> APIRVVSVPESDSFMSSVPDNSTPLYPKVVVPPRQVPGRFTNFIDVAKQTYSFCSISGKPYFEVTNTSGDEPLFQMDVSLSAAELHGTYVASLSSFFAQYRGSLNFNFIFTGAAATKAKFLVAFVPPHSAAPKTRDEAMACIHAVWD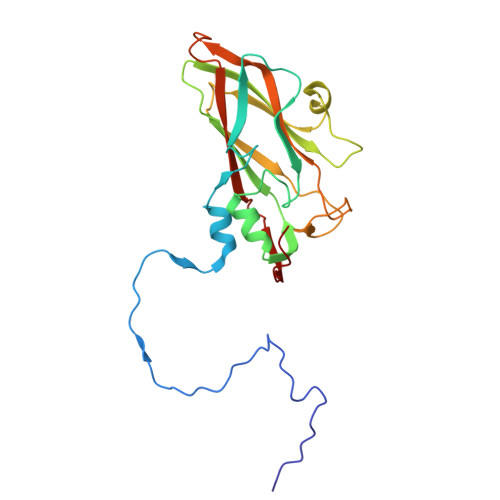VGLNSAFSFNVPYSSPADFMAVYSAEATVVNVSGWLQVYALTALTSTDIAVNSKGRVLVAVSAGPDFSLRHPVDLPDKQ~{N}-methyl-~{N}-[3-[[[2-[(2-oxidanylidene-1,3-dihydroindol-5-yl)amino]pyrimidin-4-yl]amino]methyl]pyridin-2-yl]methanesulfonamide 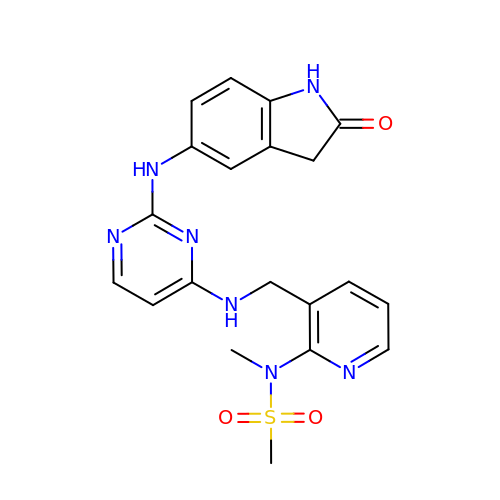| C20 H21 N7 O3 S | BTIZXJFJJCRTBP-UHFFFAOYSA-N>MTELDYQGTAEAASTSYSRNQTDLKPFPSAGSASSSIKTTEPVKDHRRRRAAAIISHVEPETFEDENDQQLLPNMNATWVDQRGAWIIHVVIIILLKLFYNLFPGVTTEWSWTLTNMTYVIGSYVMFHLIKGTPFDFNGGAYDNLTMWEQIDDETLYTPSRKFLISVPIALFLVSTHYAHYDLKLFSWNCFLTTFGAVVPKLPVTHRLRISIPGITGRAQIS[2x];>MAHIPEVLPKSIPIPAFIVTTSSYLWYYFNLVLTQIPGGQFIVSYIKKSHHDDPYRTTVEIGLILYGIIYYLSKPQQKKSLQAQKPNLSPQEIDALIEDWEPEPLVDPSATDEQSWRVAKTPVTMEMPIQNHITITRNNLQEKYTNVFNLASNNFLQLSATEPVKEVVKTTIKNYGVGACGPAGFYGNQDVHYTLEYDLAQFFGTQGSVLYGQDFCAAPSVLPAFTKRGDVIVADDQVSLPVQNALQLSRSTVYYFNHNDMNSLECLLNELTEQEKLEKLPAIPRKFIVTEGIFHNSGDLAPLPELTKLKNKYKFRLFVDETFSIGVLGATGRGLSEHFNMDRATAIDITVGSMATALGSTGGFVLGDSVMCLHQRIGSNAYCFSACLPAYTVTSVSKVLKLMDSNNDAVQTLQKLSKSLHDSFASDDSLRSYVIVTSSPVSAVLHLQLTPAYRSRKFGYTCEQLFETMSALQKKSQTNKFIEPYEEEEKFLQSIVDHALINYNVLITRNTIVLKQETLPIVPSLKICCNAAMSPEELKNACESVKQSILACCQESNK[2x];>MSTPANYTRVPLCEPEELPDDIQKENEYGTLDSPGHLYQVKSRHGKPLPEPVVDTPPYYISLLTYLNYLILIILGHVHDFLGMTFQKNKHLDLLEHDGLAPWFSNFESFYVRRIKMRIDDCFSRPTTGVPGRFIRCIDRISHNINEYFTYSGAVYPCMNLSSYNYLGFAQSKGQCTDAALESVDKYSIQSGGPRAQIGTTDLHIKAEKLVARFIGKEDALVFSMGYGTNANLFNAFLDKKCLVISDELNHTSIRTGVRLSGAAVRTFKHGDMVGLEKLIREQIVLGQPKTNRPWKKILICAEGLFSMEGTLCNLPKLVELKKKYKCYLFIDEAHSIGAMGPTGRGVCEIFGVDPKDVDILMGTFTKSFGAAGGYIAADQWIIDRLRLDLTTVSYSESMPAPVLAQTISSLQTISGEICPGQGTERLQRIAFNSRYLRLALQRLGFIVYGVADSPVIPLLLYCPSKMPAFSRMMLQRRIAVVVVAYPATPLIESRVRFCMSASLTKEDIDYLLRHVSEVGDKLNLKSNSGKSSYDGKRQRWDIEEVIRRTPEDCKDDKYFVN[2x];>MTQHKSSMVYIPTTKEAKRRNGKSEGILNTIEEVVEKLYWTYYIHLPFYLMASFDSFFLHVFFLTIFSLSFFGILKYCFL[2x]

Serine palmitoyltransferase (SPT) is the rate-limiting enzyme in the synthesis of sphingolipids. It catalyzes the transfer of a palmitoyl group to L-serine, yielding 3-ketosphinganine (3-KS). SPT is highly conserved across species and consists of two large catalytic subunits (in yeast: Lcb1 and Lcb2) and interacts with a small regulatory subunit (in yeast: Tsc3). Here, we solved cryo-EM structures of the yeast SPOT complex in both monomeric and dimeric states and the monomeric SPOTS complex.

The SPOT dimer was refined to 3.4 Å resolution, with C2-symmetry imposed. We do not observe such helix crossover for the yeast SPOT dimer. A marked difference is the absence of the previously reported crossover helices at the protomer interface in our dimeric structure, which could explain why we were able to obtain monomeric SPOT complexes. The lack of the Lcb1-TM1 helix swap, previously observed in human SPT complexes, results in weaker protomer interactions and explains the presence of monomeric complexes. Both oligomeric states from the human complexes are active in vitro; however, their respective physiological relevance is unclear. In all of our structures, TM1-2 of Orm1 acts as a docking station for a 44:0;4 ceramide, which is sandwiched between Orm1 and the amphipathic helix of Lcb2. The ceramide extends out of the cytosol-facing membrane plane through interactions with two aromatic residues, Y110 and Y485, of Lcb2. Therefore, the positioning of the 44:0;4 ceramide headgroup in the immediate proximity to the conserved, substrate-tunnel-gating PATP loop and its direct interactions with Y485 and Y110 of Lcb2 effectively blocks access to the substrate tunnel from the membrane, highlighting a regulatory mechanism of ceramide-based inhibition of SPT activity. Our data show that in yeast, Orm1 does not regulate SPT via insertion of its N-terminus into the active site but rather in conjunction with ceramide.methyl 2-(4-aminophenoxy)benzoate | 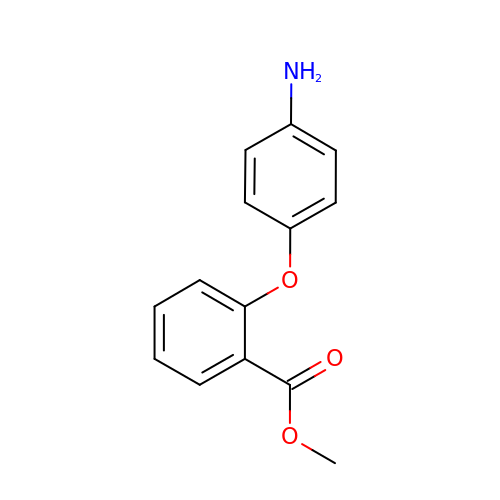C14 H13 N O3 | FXHKMQZPYDWTCS-UHFFFAOYSA-N>MRGSHHHHHHGSMAGLGHPAAFGRATHAVVRALPESLGQHALRSAKGEEVDVARAERQHQLYVGVLGSKLGLQVVELPADESLPDCVFVED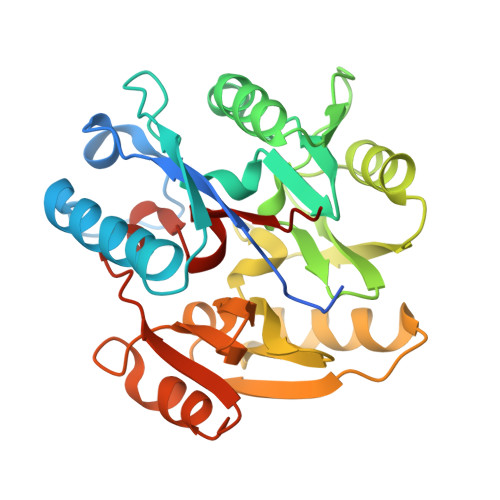VAVVCEETALITRPGAPSRRKEVDMMKEALEKLQLNIVEMKDENATLDGGDVLFTGREFFVGLSKRTNQRGAEILADTFKDYAVSTVPVADGLHLKSFCSMAGPNLIAIGSSESAQKALKIMQQMSDHRYDKLTVPDDIAANCIYLNIPNKGHVLLHRTPEEYPESAKVYEKLKDHMLIPVSMSELEKVDGLLTCCSVLINKKVDS[6x]> GGSSETQRQFSRYFIEFEELQLLGKGAFGAVIKVQNKLDGCCYAVKRIPINPASRQFRRIKGEVTLLSRLHHENIVRYYNAWIENGCHES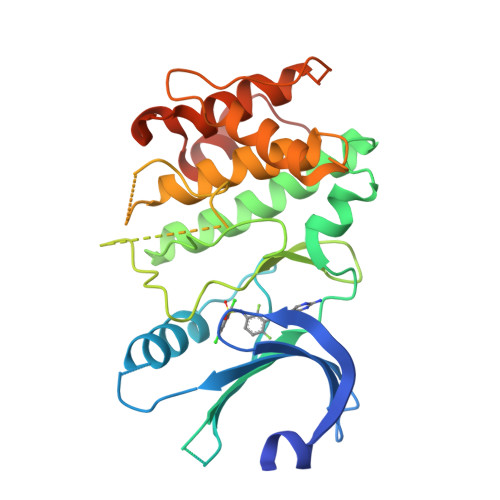EPSVTTEAVHYLYIQMEYCEASTLRDTIDQGLYRDTVRLWRLFREILDGLAYIHEKGMIHRNLKPVNIFLDSDDHVKIGDFGLATDHLAFSADSKQDDQTGDLIKSDPSGHLEGMVGEALYVSPEVQGSTKSAYNQKVDLFSLGIIFFEMSYHPMVTASERIFVLNQLRDPTSPKFPEDFDDGEHAKQKSVISWLLNHDPAKRPTATELLKSELLPPPQMEESELHE>[2x]GPGSMSKDVTPWDVNINNEEGINYNKLIKEFGCSKITENHIKRIEKLTNSKAHHFIRRGIFFSHRDLDFLLNYYEQHKCFYIYTGRGPSSLSMHLGHLIPFYFCKYLQEAFNVPLVIQ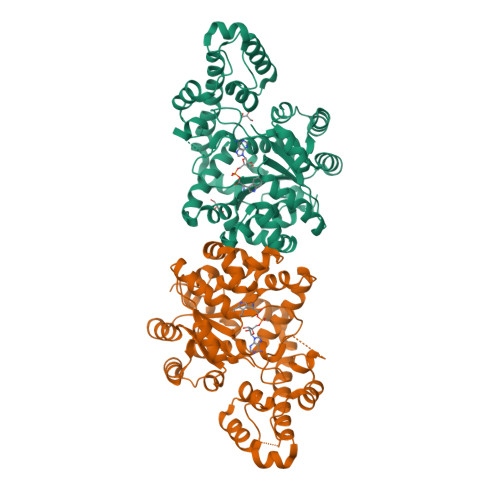LSDDEKYLFNQNYSLEYINTLTNENVKDIISVGLNPELTFIFKNTEYAGYLYPTVLSIHKKTTLNQSMNVFGFNHSDNIGKISYPSFQIAPCFSQCFPNFLGKNIPCLVPQGIDQDPYFRLSRDIAVKMALHKPVVVHSVFMPGLQGVNSKMSSTKKKKDDNGKSNSTFDHNNSVIFLTDTPEQIKNKINKYAFSGGGTTIQEHREKGGNLDKDISYQYLRYLLEDDNKLNEIGEKYKKGEMLSGEIKKILIDVLTELVLKHQEKKKSLTDEEISYFFDPNKPSLQKFKNM>GPGSSDSKQHIEVLKESLTAKEQRAAILQTEVDA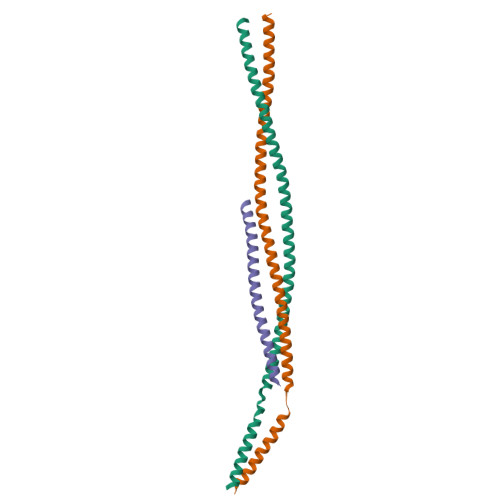LRLRLEEKETMLNKKTKQIQDMAEEKGTQAGEIHDLKDMLDVKERKVNVLQKKIENLQEQLRDKEKQMSSLKERVKSLQADTTNTDTALTTLEEALADKERTIERLKEQRDR[2x];> GPGSNTMARAKILQDIDRELDLVERESAKLRKKQAELDEEEKEIDAKLRYLEMGINRRKEALLKEREKRERAYLQGVAEDRDYMSDSEVSS> MSAEKLFTPLKVGAVTAPNRVFMAPITRLRSIEPGDIPTPLMGEYYRQRASAGLIISEATQISAQAKGYAGAPGLHSPEQIAAWKKITAGVHAEDGRIAVQLWHTGRISHSSIQPGGQAPVSASALNANTRTSLRDENGNAIRVDTTTPRALELDEIPGIVNDFRQAVANAREAGFDLVELHSAHGYLLHQFLSPSSNQRTDQYGGSVENRARLVLEVVDAVCNEWSADRIGIRVSPIGTFQNVDNGPNEEADALYLIEELAKRGIAYLHMSETDLAGGKPYSEAFRQKVRERFHGVIIGAGAYTAEKAEDLIGK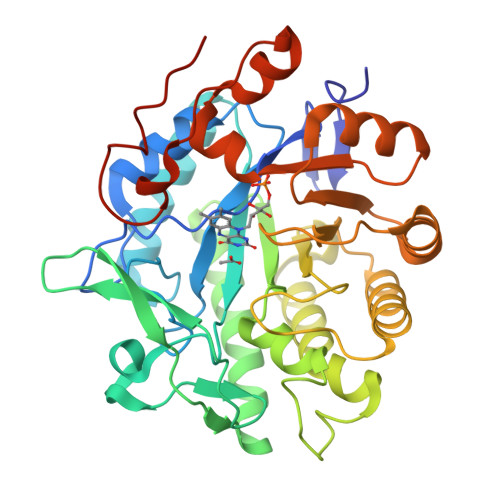GLIDAVAFGRDYIANPDLVARLQKKAELNPQRPESFYGGGAEGYTDYPSLHHHHHHHH>MARIIVVTSGKGGVGKTTSSAAIATGLAQKGKKTVVIDFAIGLRNLDLIMGCERRVVYDFVNVIQGDATLNQALIKDKRTENLYILPASQTRDKDALTREGVAKVLDDLKAMDFEFIVCDSPAGIETGALMALYFADEAIITTNPEVSSVRDSDRILGILASKSRRAENGEEPIKEHLLLTRYNPGRVSRGDMLSMEDVLEILRIKLVGVIPEDQ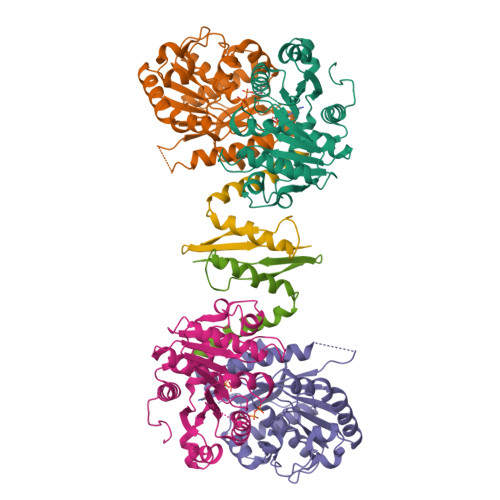SVLRASNQGEPVILDINADAGKAYADTVERLLGEERPFRFIEEEK[2x];>[2x]KNTANIAKERLQNIVAERRRSDAEPHYLPQLRKDILEVICKYVQIDPEMVTVQLEQKDGDISILELNVTLPEAEELK ATM/Tel1 belongs to the evolutionarily conserved phosphatidylinositol-3-kinase-related protein kinase (PIKK) family. In budding yeast, Tel1 and Mec1 correspond to ATM and ATR, respectively. ATM primarily responds to DNA double-strand breaks (DSBs), whereas ATR is activated by DSBs as well as various types of DNA replication stress. Under normal cellular conditions, ATM is inactive and exists in a homodimeric form.

Besides the 4.1 Å cryo-EM structure of symmetric dimer, we also determined a 4.3 Å structure of asymmetric dimer of Tel1/ATM, which allows to trace the course of the polypeptide. We next compared the Tel1 structures of the Compact and Butterfly conformers. In the Compact Tel1, the FAT and kinase N-lobe move down by ~5–8 Å, whereas the Spiral of α-solenoid moves upwards by ~11 Å relative to their positions in the Butterfly conformer. The overall height has been reduced from 190 Å (Butterfly) to 175 Å (Compact). The kα11 and kα12 (FATC) are partially disordered, while the α4 (TRD2), α15 (TRD3) and kα9b (PRD) are almost fully disordered in the Compact conformer. As the PRD and FATC become disordered, their inhibition on the activation loop is at least partially relieved, which can now move outside of the substrate-binding groove by ~6 Å. However, the disordered fragments in the Compact monomer release these constraints, leaving sufficient space for a peptide substrate to bind. The activation loop could move outside of the substrate-binding groove to access substrates in the Compact conformer.

> MEDHGIVETLNFLSSTKIKERNNALDELTTILKEDPERIPTKALSTTAEALVELLASEHTKYCDLLRNLTVSTTNKLSLSENRLSTISYVLRLFVEKSCERFKVKTLKLLLAVVPELMVKDGSKSLLDAVSVHLSFALDALIKSDPFKLKFMIHQWISLVDKICEYFQSQMKLSMVDKTLTNFISILLNLLALDTVGIFQVTRTITWTVIDFLRLSKKENGNTRLIMSLINQLILKCHCFSVIDTLMLIKEAWSYNLTIGCTSNELVQDQLSLFDVMSSELMNHKLPYMIGQENYVEELRSESLVSLYREYILLRLSNYKPQLFTVNHVEFSYIRGSRDKNSWFALPDFRLRDRGGRSVWLKILGITKSLLTYFALNRKNENYSLLFKRRKCDSDIPSILRISDDMDTFLIHLLEENSSHEFEVLGLQLCSFYGTLQDFTKSFAEQLKELLFSKFEKIQCFNWVCFSFIPLLSQKECELSNGDMARLFKVCLPLVKSNESCQLSCLLLANSIKFSKQLLSDEKTINQIYDLYELSDILGPILVTNESFMLWGYLQYVGKDFQSMNGISSADRIFEWLKSKWNQLRGTDAKQDQFCNFISWLGNKYDPENPFNDKKGEGANPVSLCWDESHKIWQHFQEQREFLLGVKPEEKSECFNTPFFNLPKVSLDLTRYNEILYRLLENIESDAFSSPLQKFTWVAKLIQIVDNLCGDSTFSEFIAAYKRTTLITIPQLSFDSQNSYQSFFEEVLSIRTINVDHLVLDKINMKEIVNDFIRMQKNKSQTGTSAINYFEASSEDTTQNNSPYTIGGRFQKPLHSTIDKAVRAYLWSSRNKSISERLVAILEFSDCVSTDVFISYLGTVCQWLKQAIGEKSSYNKILEEFTEVLGEKLLCNHYSSSNQAMLLLTSYIEAIRPQWLSYPEQPLNSDCNDILDWIISRFEDNSFTGVAPTVNLSMLLLSLLQNHDLSHGSIRGGKQRVFATFIKCLQKLDSSNIINIMNSISSYMAQVSYKNQSIIFYEIKSLFGPPQQSIEKSAFYSLAMSMLSLVSYPSLVFSLEDMMTYSGFNHTRAFIQQALNKITVAFRYQNLTELFEYCKFDLIMYWFNRTKVPTSKLEKEWDISLFGFADIHEFLGRYFVEISAIYFSQGFNQKWILDMLHAITGNGDAYLVDNSYYLCIPLAFISGGVNELIFDILPQISGKTTVKYHKKYRLLMLKWIIRFTDLGSLTELRSTVEKLFPTSYLSPYLFENSSVSMRYQYPLHIPLALGATLVQTQFAHEKNNTHEFKLLFLSVITDLEKTSTYIGKLRCARELKYLFVLYENVLVKSSTLNFIIIRLSKFLIDTQIHDEVITIFSSLLNLADKNTFEIEPSLPNLFCKIFIYLRENKQLSPSFQQAIKLLEHRDLIKIKTWKYCLDAIFGNIVQDDIYENTELLDASDCGVDDVVLVSLLFSYARRPVASKIGCSLSKAAAINILKHHVPKEYLSKNFKLWFAALSRRILQQEVQRERSTNFNNEVHLKNFEMVFRHPEQPHMIYQRISTFNKEAELYDSTEVFFISECILTYLVGYSIGNSESEFCFRDNIMNENKDKVAPLDKDVLNAIYPLANNFGMESFICDTYLSVNEPYNCWLSKFARSLIHQISFNIPPIVCLYPLCKGSTAFCELVLTDLFFLSTTYDPKSCLNWSNRIFTQIAMLLHVKDSEIKLKMLFNVIKMIRMGSRCKERNCLRIYSSLDLQEICQISLKIKEFKFGYLLFEEMNMPNIREMNINTLQKIYECINDGDFLAGLPVPHSIEGVLNSINRIDSDTWKRFLFNNADFDANYTTSLEEEKESLIKATEDSGFYGLTSLLESRLSGSSDVYKWNLELGDWKLLTPKVVDSKAKGLYYAIKNLPQDVGFAEKSLEKSLLTIFDSRQHFISQTEWMDTLNAIIEFIKIAAIPQDVTSFPQTLMSIMKADKERLNTIDFYDHKTTLKSRHTLMNVLSRNSLDENVKCSKYLRLGSIIQLANYVQLAIANGAPQDALRNATLMSKTVKNIAKLYDDPSVVSQIEKLASFTSANALWESREYKAPVMIMRDLLAQNEKNISESILYDDFKLLINVPMDQIKARLVKWSSESRLEPAAAIYEKIIVNWDINVEDHESCSDVFYTLGSFLDEQAQKLRSNGEIEDREHRSYTGKSTLKALELIYKNTKLPENERKDAKRHYNRVLLQYNRDSEVLKALLLQKEKFLWHALHFYLNTLVFSNRYDNDIIDKFCGLWFENDDNSKINQLLYKEIGTIPSWKFLPWVNQIASKISMEENEFQKPLQLTMKRLLYKLPYDSLYSVMSILLYEKQSNKDTNISQKIQAVKKILLELQGYDRGAFAKKYLLPVQEFCEMSVELANLKFVQNTKTLRLANLKIGQYWLKQLNMEKLPLPTSNFTVKSSADGRKARPYIVSVNETVGITTTGLSLPKIVTFNISDGTTQKALMKGSNDDLRQDAIMEQVFQQVNKVLQNDKVLRNLDLGIRTYKVVPLGPKAGIIEFVANSTSLHQILSKLHTNDKITFDQARKGMKAVQTKSNEERLKAYLKITNEIKPQLRNFFFDSFPDPLDWFEAKKTYTKGVAASSIVGYILGLGDRHLNNILLDCSTGEPIHIDLGIAFDQGKLLPIPELVPFRLTRDIVDGFGVTGVDGLFRRSCERVYAVLRKDYVKVMCVLNILKWDPLYSWVMSPVKKYEHLFEEEHEITNFDNVSKFISNNDRNENQESYRALKGVEEKLMGNGLSVESSVQDLIQQATDPSNLSVIYMGWSPFY>MNHLGKTEVFLNRFALRPLNPEELRPWRLEVVLDPPPGREEVYPLLAQVARRAGGVTVRMGDGLASWSPPEVLVLEGTLARMGQTYAYRLYPKGRRPLDPKDPGERSVLSALARRLLQERLRRLEGVWVEGLAVYRREHARGPGWRVLGGAVLDLWVSDSGAFLLEVDPAYRILCEMSLEAWLAQGHPLPKRVRNAYDRRTWELLRLGEEDPKELPLPGGLSLLDYHASKGRLQGREGGRVAWVADPKDPRKPIPHLTGLLVPVLTLEDLHEEEGSLALSLPWEERRRRTREIASWIGRRLGLGTPEAVRAQAYRLSIPKLMGRRAVSKPADALRVGFYRAQETALALLRLDGAQGWPEFLRRALLRAFGASGASLRLHTLHAHPSQGLAFREALRKAKEEGVQAVLVLTPPMAWEDRNRLKALLLREGLPSQILNVPLREEERHRWENALLGLLAKAGLQVVALSGAYPAELAVGFDAGGRESFRFGGAACAVGGDGGHLLWTLPEAQAGERIPQEVVWDLLEETLWAFRRKAGRLPSRVLLLRNGR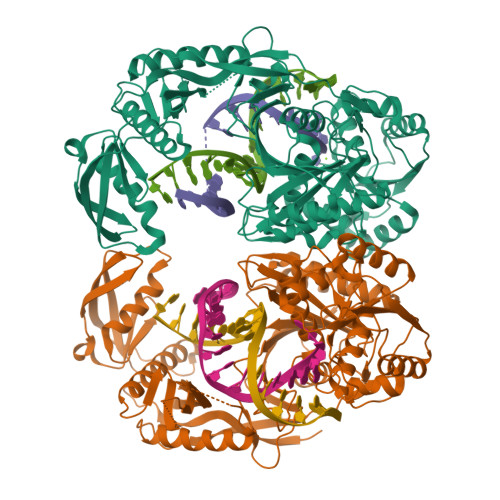VPQDEFALALEALAREGIAYDLVSVRKSGGGRVYPVQGRLADGLYVPLEDKTFLLLTVHRDFRGTPRPLKLVHEAGDTPLEALAHQIFHLTRLYPASGFAFPRLPAPLHLADRLVKEVGRLGIRHLKEVDREKLFFV[2x]>[4x]MKQKVVSIGDINVANDLPFVLFGGMNVLESRDLAMRICEHYVTVTQKLGIPYVFKASFDKANRSSIHSYRGPGLEEGMKIFQELKQTFGVKIITDVHEPSQAQPVADVVDVIQLPAFLARQTDLVEAMAKTGAVINVKKPQFVSPGQMGNIVDKFKEGGNEKVIL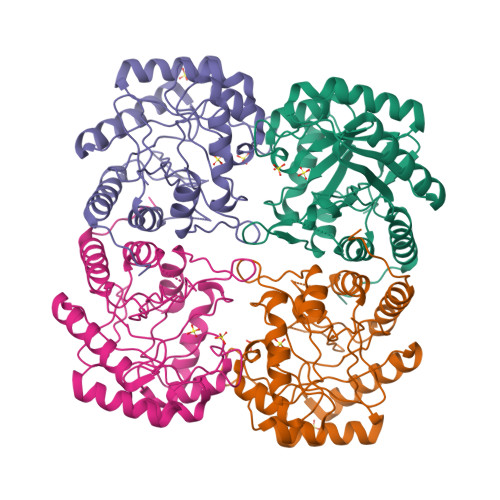CDRGANFGYDNLVVDMLGFSIMKKVSGNSPVIFDVTHALQCRDPFGAASGGRRAQVAELARAGMAVGLAGLFIEAHPDPEHAKCDGPSALPLAKLEPFLKQMKAIDDLVKGFEELDTSK> VTNVGEDGEPGETEPRHALSPVDMHVHTDVSFLLDRFFDVETLELSNLTGSPATHVLDPFGSTAQLAWARLLNTCTYFFSDLELSIQFKFTTTPSSVGEGFVWVKWFPVGAPTKTTDAWQLEGGGNSVRIQQLAVAGMSPTVVFKIAGSRSQACGFSVPYTSMWRVVPVFYNGWGAPTKEKATYNWLPGAHFGSILLTSDAHDKGGCYLRYRFPRANMYCPRPIPPAFTRPADKTRHKFPTNINKQCT;> DKKTEETTNIEDRIETTVVGATIINSQGSVGTTYCYSKPDG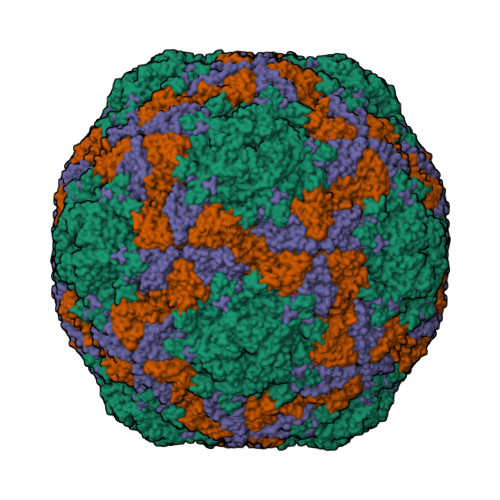RPPSTVSDPVTRLGPTLSRHYTFKVGEWPHSQSHGHAWICPLPSDKLKKMGSFHEVVKAHHLVKNGWDVVVQVNASFAHSGALCVAAVPEYEHTHEKALKWSELEEPAYTYQQLSVFPHQLLNLRTNSSVHLVMPYIGPGPTTNLTLHNPWTIVILILSELTGPGQTVPVTMSVAPIDAMVNGPLPNPE;> APIRVVSVPESDSFMSSVPDNSTPLYPKVVVPPRQVPGRFTNFIDVAKQTYSFCSISGKPYFEVTNTSGDEPLFQMDVSLSAAELHGTYVASLSSFFAQYRGSLNFYFIFTGAAATKAKFLVAFVPPHSAAPKTRDEAMACIHAVWDVGLNSAFSFNVPYSSPADFMAVYSAEATVVNVSGWLQVYALTALTSTDIAVNSKGRVLVAVSAGPDFSLRHPVDLPDKQ;> GAGTSTPTTGNQNMSGNSGSIVQNFYMQQYQNSIDADLGDNVISPEGQGSNTSSSTSSSQSSGLGGWFSSLLNLGTKLLA>[2x]MSMAEMLRRDEGLRLKVYWDTEGYPTIGIGHLIMKQPVRDMAQINKVLSKQVGREITGNPGSITMEEATTLFERDLADMQRDIKSHS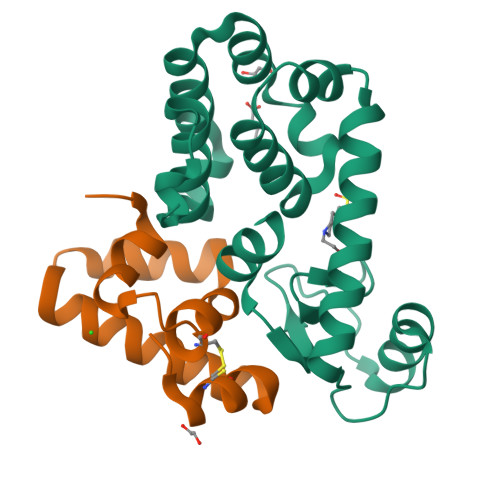KVGPVWQAVNRSRQMALENMAFQMGVGGVAKFNTMLTAMLAGDWEKAYKAGRDSLWYQQTKGRASRVTMIILTGNLESYGVELEHHHHHH;>MKKFIFATIFALASCAAQPAMAGYDKDLCEWSMTADQTEVETQIEADIMNIVKRDRPEMKAEVQKQLKSGGVMQYNYVLYCDKNFNNKNIIAEVVGELEHHHHHH[2x]> MAKQYDDNECPFCDEVSKYEKLAKIGQGTFGEVFKARHRKTGQRVALKKVLMENEKEGFPITALREIKILQLLKHENVVNLIEICRTKASPYNRCKGSIYLVFDFCEHDLAGLLSNVLVKFTLSEIKRVMQMLLNGLFYIHRNKILHRDMKAANVLITRDGVLKLADFGLARAFSLAKNSQPNRYTNRVVTLWYRPPELLLGERDYGPPIDLWGAGCIMAEMWTRSPIMQGNTEQHQLALISQLCGSITPEVWPNVDNYELYEKLELVKGQKRKVKDRLAAYVRDPYALDLIDKLLVLDPAQRIDSEDALEHDFFWSDPMPSDLKGMLST;> MEGERKNNNKRWYFT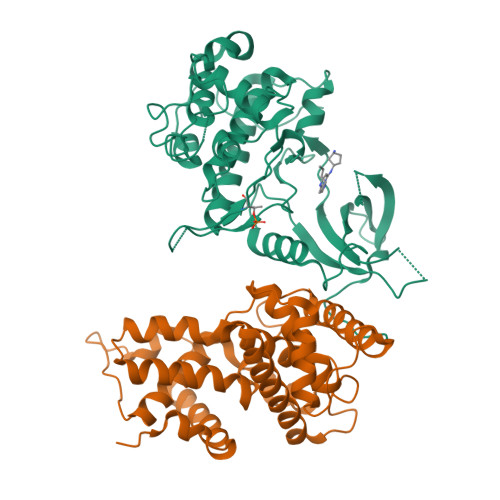REQLENSPSRAFGVDPDKELSYRQQAANLLQDMGQRLNVSQLTINTAIVYMHRFYMIQSFTRFPGNSVAPAALFLAAKVEGQPKKLEHVIRVAHTCLHPQESLPDTRSEAYLQQVQDLVILESIILQTLGFELTIDHPHTHVVKCTQLVRASKDLAQTSYFMATNSLHLTTFSLQYTPPVVACVCIHLACKWSNWEIPVSTDGKHWWEYVDATVTLELLDELTHELLQILEKTPNRLKRIWNWR> GAMDARSVN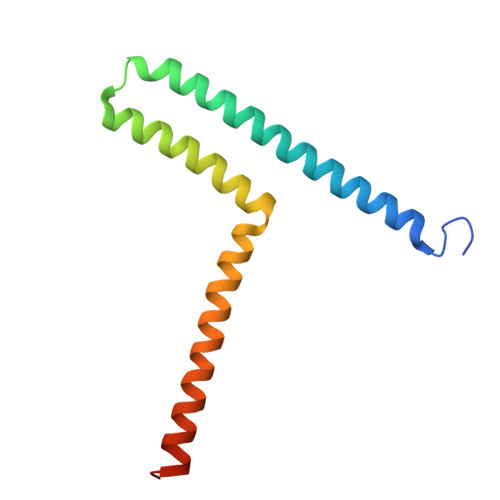GEFPRHVKLKNEIENLLDQVTQLYTKHNSNYQQYNAQAGRLDLRQKAEYLKGLNDWAERLLQELNGEDVKKVLGKVAFEKDDLEKEVKELKEKIDKKEKEYQDC>MKTSDFVKYLQRMIAITDTGLTFTKDPFDRERYEDLRSLLSEMLNQASDLDSEEVAEVLKPTSAYATPLMDVRAWIVEDEKICLVRGQGEDSWALPGGFGEVGYSPTENILKEIEEETGFKAKVERLLAVFDTNRFQLQSKQYTKF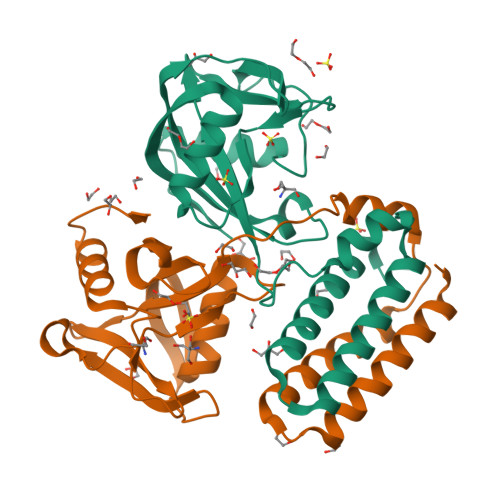VFGCKLLDGQFQENQEIADLQFFAIDQLPNLSEKRITKEQIELLWQVYQGHRGQYLD[2x]> MARENGESSSSWKKQAEDIKKIFEFKETLGTGAFSEVVLAEEKATGKLFAVKCIPKKALKGKESSIENEIAVLRKIKHENIVALEDIYESPNHLYLVMQLVSGGELFDRIVEKGFYTEKDASTLIRQVLDAVYYLHRMGIVHRDLKPENLLYYSQDEESKIMISDFGLSKMEGKGDVMSTACGTPGYVAPEVLAQKPYSKAVDCWSIGVIAYILLCGYPPFYDENDSKLFEQILKAEYEFDSPYWDDISDSAKDFIRNLMEKDPNKRYTCEQAARHPWIAGDTALNKNIHESVSAQIRKNFAKSKWRQAFNATAVVRHMRKLHLGSSLDSSNASVSSSLSLASQKDCLAPSTLCSFISSSSGVSGVGAE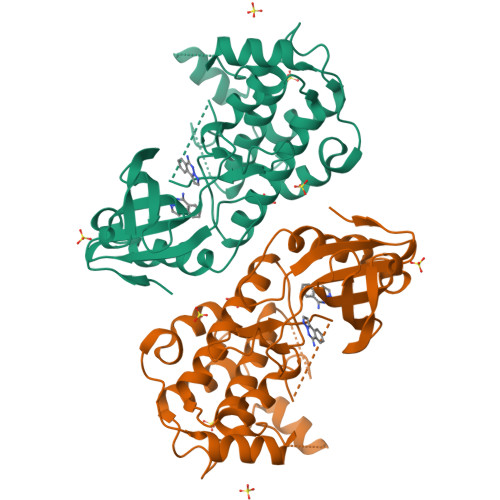RRPRPTTVTAVHSGSK>GLTYSQTMELKDSMLQLDPNAKTWIDIEGRPEDPVEIAIYQPNNGQYIHFYREPTDIKQFKQDSKHSHGIDIQDLFSVQPGLTSAVIESLPKNMVLSCQGADDIRKLLDSQNRRDIKLIDVSMQKDDARKFEDKIWDEYKHLCRMHTGIVTQKKKRGGKEEVTPHCALLDCLMFEAAVIGSPQIPTPRPVLS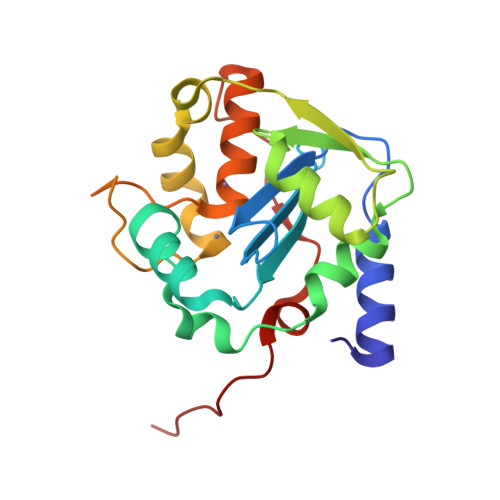RDLVFRTGPPRVVL[2x]propan-2-yl N-[(2S)-1-oxidanylidene-1-[[(2S)-1-oxidanyl-3-[(3S)-2-oxidanylidenepyrrolidin-3-yl]propan-2-yl]amino]-3-phenyl-propan-2-yl]carbamate 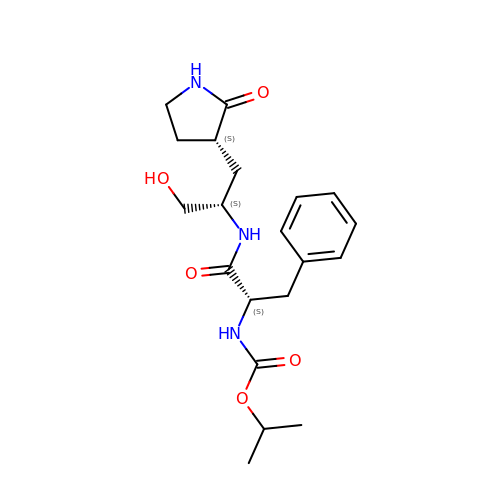| C20 H29 N3 O5 | DESRATCONZEYFJ-ULQDDVLXSA-N>[2x]GSGAAGTTTTSVTVHKLLATDGDMDKIANELETGNYAGNKVGVLPANAKEIAGVMFVWTNTNNEIIDENGQTLGVNIDPQTFKLSGAMPATAMKKLTEAEGAKFNTANLPAAKYKIYEIHSLSTYVGEDGATLTGSKAVPIEIELPLNDVVDAHVYPKNTEAKPKIDKDFKGKANPDTPRVDKDTPVNHQVGDVVEYEIVTKIPALANYATANWSDRMTEGLAFNKGTVKVTVDDVALEAGDYALTEVATGF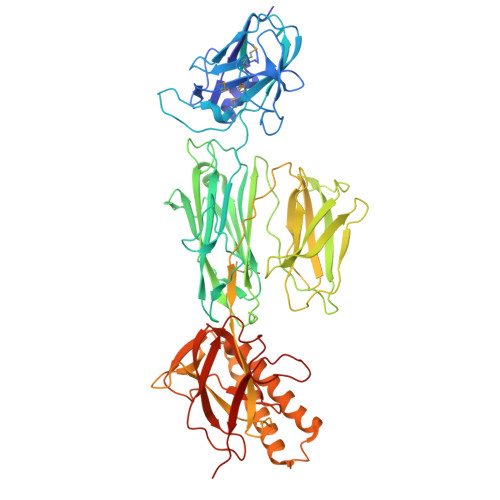DLKLTDAGLAKVNDQNAEKTVKITYSATLNDKAIVEVPESNDVTFNYGNNPDHGNTPKPNKPNENGDLTLTKTWVDATGAPIPAGAEATFDLVNAQTGKVVQTVTLTTDKNTVTVNGLDKNTEYKFVERSIKGYSADYQEITTAGEIAVKNWKDENPKPLDPTEPKVVTYGKKFVKVNDKDNRLAGAEFVIANADNAGQYLARKADKVSQEEKQLVVTTKDALDRAVAAYNALTAQQQTQQEKEKVDKAQAAYNAAVIAANNAFEWVADKDNENVVKLVSDAQGRFEITGLLAGTYYLEETKQPAGYALLTSRQKFEVTATSYSATGQGIEYTAGSGKDDATKVVNKKITI> GQRESKEALEIEKNSRKPPPYKHIKANKVIGKVQIQVADLSEIPRCNCKPADENPCGLESECLNRMLQYECHPQVCPAGDRCQNQCFTKRLYPDAEIIKTERRGWGLRTKRSIKKGEFVNEYVGELIDEEECRLRIKRAHENSVTNFYMLT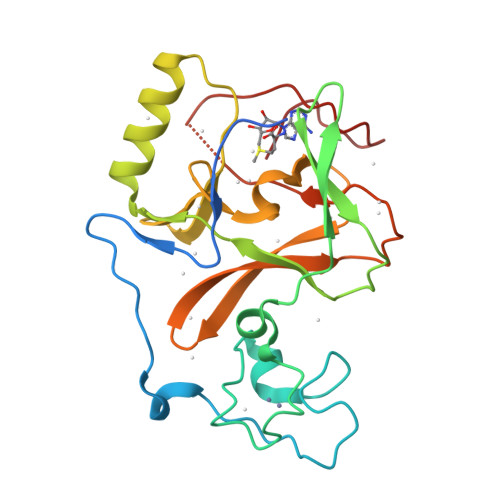VTKDRIIDAGPKGNYSRFMNHSCNPNCETQKWTVNGDVRVGLFALCDIPAGMELTFNYNLDCLGNGRTECHCGADNCSGFLG>[2x]GPGSELPQMVQQLNSPDQQELQSALRKLSQIASGGNEQIQAVIDAGALPALVQLLSSPNEQILQEALWALSNIASGGNEQIQAVIDAGALPALVQLLSSPNEQ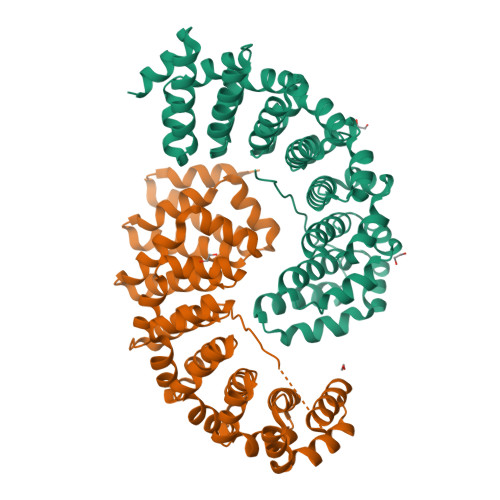ILQEALRALQQIAMGGNEQIQAVIDAGALPALVQLLSSPNEQILASALGALANIASGGNEQIQAVIDAGALPALVQLLSSPNEQILQFALIALSNIASGGNEQIQAVIDAGALPALVQLLSSPNEQILQEALWALSNIASGGNEQIQAVIDAGALPALVQLLSSPNEQILQEALWALSNIASGGNEQKQAVKEAGALEKLEQLQSHENEKIQKEAQEALEKLQSHGSGGSGKRKAKITWKR> DLGTFYREFQNPPQLSSLSIDIGAQSMAEDLDSLPEKLAVHEKNVREFDAFVETLQ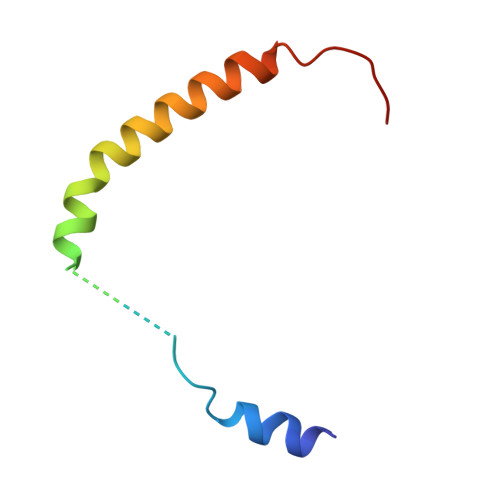GSDEA>EPEWTYPRLSCQGSTFQKALLISPHRFGEARGNSAPLIIREPFIACGPKECKHFALTHYAAQPGGYYNGTREDRNKLRHLISVKLGKIPTVENSIFHMAAWSGSACHDGREWTYIGVDGPDSNALIKIKYGEAYTDTYHSYANNILRTQESACNCIGGDCYLMITDGSASGISKCRFLK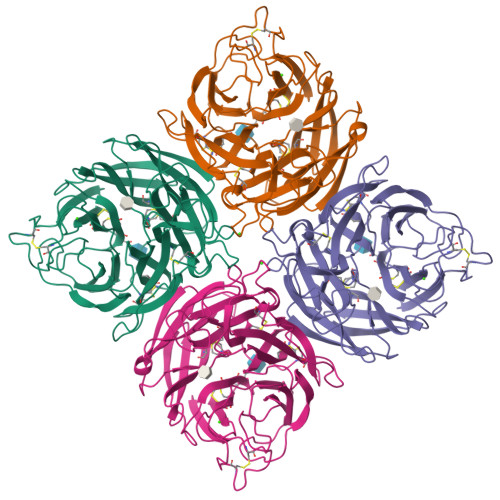IREGRIIKEIFPTGRVEHTEECTCGFASNKTIECACRDNSYTAKRPFVKLNVETDTAEIRLMCTETYLDTPRPDDGSITGPCESNGDKGRGGIKGGFVHQRMASKIGRWYSRTMSKTERMGMELYVRYDGDPWTDSDALAHSGVMVSMKEPGWYSFGFEIKDKKCDVPCIGIEMVHDGGKKTWHSAATAIYCLMGSGQLLWDTVTGVDMAL[2x]> MHGRLKVKTSEEQ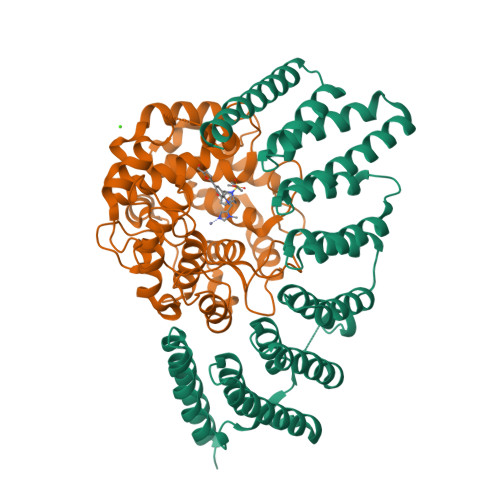AEAKRLEREQKLKLYQSATQAVFQKRQAGELDESVLELTSQILGANPDFATLWNCRREVLQHLETEKSPEESAALVKAELGFLESCLRVNPKSYGTWHHRCWLLSRLPEPNWARELELCARFLEADERNFHCWDYRRFVAAQAAVAPAEELAFTDSLITRNFSNYSSWHYRSCLLPQLHPQPDSGPQGRLPENVLLKELELVQNAFFTDPNDQSAWFYHRWLLGAGSGRCELSVEKSTVLQSELESCKELQELEPENKWCLLTIILLMRALDPLLYEKETLQYFSTLKAVDPMRAAYLDDLRSKFLLENSVLKMEYA;> GTQQKDVTIKSDAPDTLLLEKHADYIASYGSKKDDYEYCMSEYLRMSGVYWGLTVMDLMGQLHRMNKEEILVFIKSCQHECGGVSASIGHDPHLLYTLSAVQILTLYDSIHVINVDKVVAYVQSLQKEDGSFAGDIWGEIDTRFSFCAVATLALLGKLDAINVEKAIEFVLSCMNFDGGFGCRPGSESHAGQIYCCTGFLAITSQLHQVNSDLLGWWLCERQLPSGGLNGRPEKLPDVCYSWWVLASLKIIGRLHWIDREKLRSFILACQDEETGGFADRPGDMVDPFHTLFGIAGLSLLGEEQIKPVSPVFCMPEEVLQRVNVQPELVS> MAHHHHHHMINITLPDGSRREFENPVSVMEVAQSIGAGLAKATIAGAVDGVLVDASDVIDHDASLRIITAKDEEGVEIIRHSCAHLVGHAVKQLYPDVKMVIGPVIAEGFYYDIYSERPFTPDDMAAIEKRMGELIAQDYDVIKKMTPRAEVIEIFKARGEDYKLRLIEDMSEDIQAMGMYYHQEYVDMCRGPHVPNTRFLKAFKLTRISGAYWRGDAQNEQLQRIYGTAWADKKQLEAYIKRIEEAEMRDHRRI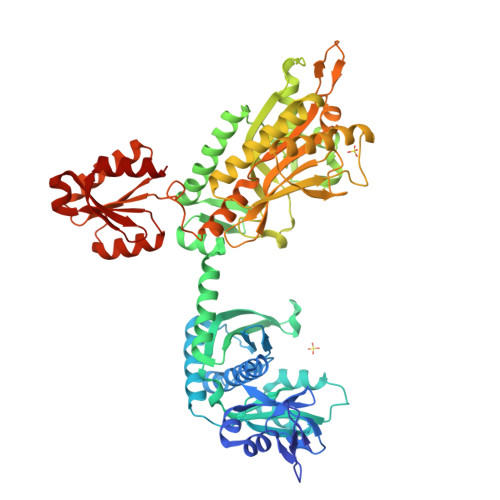GKQQDLFHLQEEAPGLVFWHPKGWALWQVVEQYMRKVYRNSGYGEVRCPQILDVSLWKKSGHWDNYQDNMFFTESEKRTYAVKPMNCPGHIQVFNQGLHSYRDLPIRYGEFGSCHRNEPSGALHGILRVRGFTQDDGHVFCTENQIESEVTAFHQQALAVYQHFGFDEIQIKIALRPESRLGDDATWDKAEGALRSALTACGVEWQELPGEGAFYGPKIEYHLKDAIGRTWQLGTMQVDFMMPGRLGAEYVDENSQKKHPVMLHRAIVGSMERFLGILIEHHAGQFPAWLAPTQVVVANITDAQADYVSGVTKTLAEQGFRVSSDLRNEKIGYKIREHTLQRVPYLLVIGDREKENGAVAVRTRSGEDLGSMSLQAFIERLHAEGA>GPKLLQILNVRVVGSGERVVVLSHGFGTDQSAWSRVLPYLTRDHRVVLYDLVCAGSVNPDHFDFRRYDNLDAYVDDLLAILDALRIPRCAFVGHSVSAMIGILASIRRPDLFAKLVLIGASPRFLNDSDYHGGFELEEIQ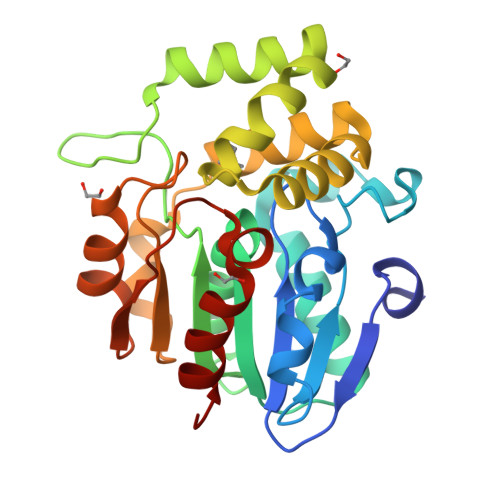QVFDAMGANYSAWATGYAPLAVGADVPAAVQEFSRTLFNMRPDISLHVCQTVFKTDLRGVLGMVRAPCVVVQTTRDVSVPASVAAYLKAHLGGRTTVEFLQTEGHLPHLSAPSLLAQVLRRALARY[2x]>MTVLATSRLHIEGDFRGYGSLDKSPPGALETLNRLMQNNHDEFDMFWRPDAGHNHTAHSLLSVYALGGSSADLERAYRDDDPHQVPIGAVDHSVVASLKDPRIFIHRMQRLDQYSNYLRFFEERIEARGWKAVVVEYLFSRSDAAEAMLGQLFEGAYHPLIQLGFGIEFELPGLVAEGLAHCAAHDAANIIPFFQKAEKLAKSGSVAPAPLVELYKEVRDTEKIRLAAKMTQGPVRVRDGVMGEAQDDIAAVAAKFQVGPDGLKQAIIETTSCAAYSCGGAQRPGKVAKVDFFFMHMVTSSIFLSILARQDWLETEDKIRLVEWKGRLDLVWYAASSAPALDRKWLEQYQPTLSAGMDWRALYRAVTVEPDD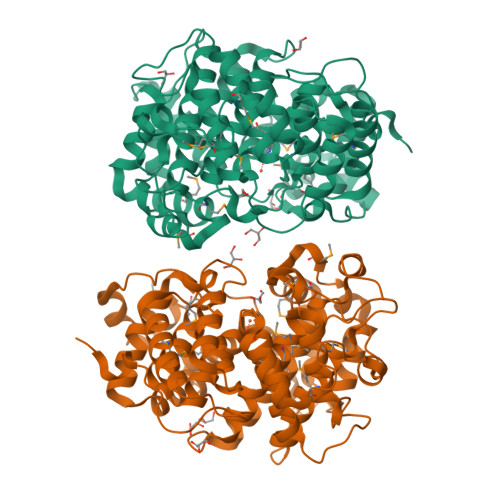GHLAKIVRSLKWAEEEAKGVETSETIPVAGSGWFKLAQMAYDSTAHLPIPAKWIMGAGYDFLWTRVDSLPAA[2x]> MVEMGRREEMIAKIKELMLQPERIRNIGIAAHIDHGKTTLSDNLLAGAGMISEELAGKQLVLDFDEQEQARGITINAANVSMVHNYEGKDYLINLIDTPGHVDFGGDVTRAMRAIDGVIIVVDAVEGVMPQTETVVRQALREYVKPVLFINKVDRLIRELKLTPQQMMERFSKIIMDVNRLIQRYAPEEYKKKWMVKVEDGSVAFGSAYYNWALSVPFMKRTGVKFNEIIDLTLKGDNRTLRQKAPLHVVVLDMVVRHLPSPIEAQKYRIPHLWE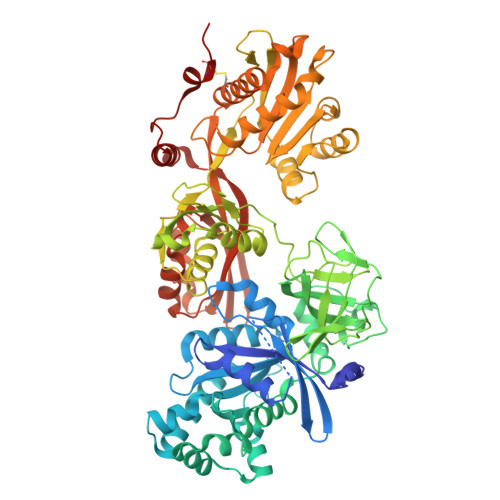GDISSDIGQAMLNCDPKGKMVMVVTKIIIDKHAGEVATGRVWSGTVKSGQEVYLINTKRKARIQQVGIYMGPERINMEAVPAGNIVAVTGLRDAMAGETVAEEQIEPFEALHYVSEPVVTVAIEAKNVKDLPRLIEALRQLAKEDPTLHVKIDEETGQHLLSGMGELHLEVKLYKLKKDWGIDIEVSEPIVVYRESITKSSPMVEGKSPNRHNRFYIVVEPMPDEIYNAIKEGIIPEGRVKNPKEVAKKLAELGMDYEIARGIVDIYNGNMFIDNTKGVQYLNEVMDLLIDGFHQAMDEGPLAREPVMKVIVRLLDAQVHEDNVHRGPAQIYPAIRTAIHCAMMKSNPVLYEPYQKVIINIPYEYMGAVSREITQRRGQLVDMKQEGEVMTIIAEAPVAEMFGFAGSIRSATSGRALWSTEHAGFKRVPNELAQQIIRQIRQRKGLDPNPPTEKDVCPLFLEHHHHHH3-[7,8-dimethyl-2,4-bis(oxidanylidene)benzo[g]pteridin-10-yl]propylcarbamic 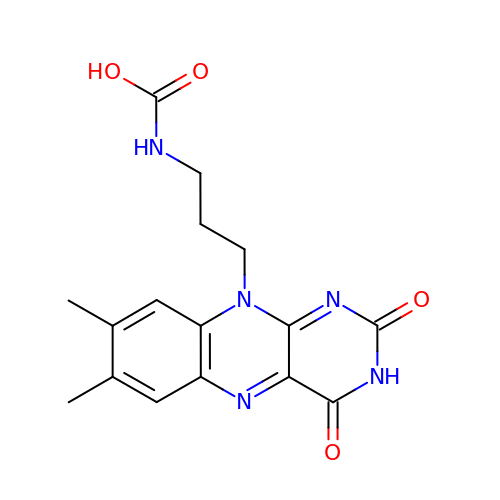acid | C16 H17 N5 O4 | SDVCPFDZIJESAH-UHFFFAOYSA-N> MSGVKVRREDAKKVLELLKSVGILDGKRKAIRDEKYVIFPVTDTNIAKSLGLEVVDVELPMRPERQIYKNLEDLLPREIFKKLGRLDIVGDIAIVSIPDEILSEREVIVSAIRKLYPKVKVIARRGFHSGLYRIRELEVIWGENRLHTIHKENGVLIKVDLSKVFFNPRMKGERYRIAQLVNDGERILVPFAGVIPYPLVIARFKNVEVYAVEINEFAVKLAEENLELNRDRLKGKIKIIHGDVFEVL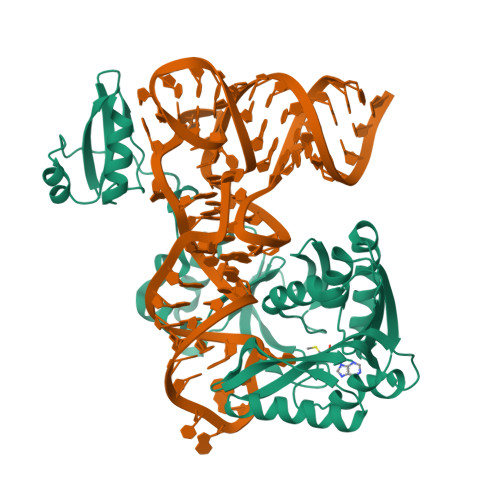PNLPNFDRVVSPTPKGVDALSLTLSKAEKFLHYYDFVHESEIERFRERVLEECRRQGKECRVSVRKVSDYKPHVYKVCADVEILS PF-3463275 | C19 H22 Cl F 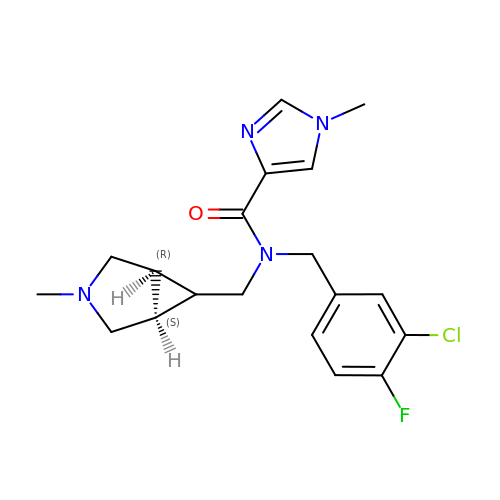N4 O | KYLOBHXXQOZRKK-QDMKHBRRSA-N>[6x]GPAGSMKPQIRNMVEPMDPRTFVSNFNNRPILSGLDTVWLCCEVKTKDPSGPPLDAKIFQGKVYPKAKYHPEMRFLRWFHKWRQLHHDQEYKVTWYVSWSPCTRCANSVATFLAKDPKVTLTIFVARLYYFWKPDYQQALRILAEAGATMKIMNYNEFQDCWNKFVDGRGKPFKPWNNLPKHYTLLQATLGELLRH

APOBEC3s (A3s) are deoxycytidine deaminases that have important roles in mammalian innate immune responses. Members of this family catalyze the conversion of cytosine into uracil on single-stranded DNA (ssDNA) and restrict retroviral replication and endogenous retroelements. Among all the A3s, A3G is most known for being a potent restriction factor against HIV-1. Similar to hA3G-CD1, rA3G-CD1 forms oligomers, binds to ssDNA/RNA strongly, and is catalytically inactive.

Here, we report the high-resolution (2 Å) crystal structure of a nearly wild-type (WT) A3G-CD1 from rhesus macaque (Macaca mulatta) (rA3G-CD1). We obtained two crystal forms of the rA3G-CD1 protein under different crystallization conditions, and determined the structures to 2 Å (CD1-1) in one crystal form and 2.9 Å (CD1-2) in the other crystal form, each in different space groups and with different crystal packing interactions. However, these two structures are essentially the same, with a Cα r.m.s. deviation of about 0.54 Å, indicating that the structures from the two different crystal forms, including the surface loops, are not affected by different crystal packing or buffer conditions. Therefore, the 2 Å high-resolution structure CD1-1 was used for structural analysis and comparison with other A3s, as similar results were also seen with the 2.9 Å resolution structure CD1-2. The 2 Å crystal structure of rA3G-CD1 indicates that the core structures of both the non-catalytic CD1 and the catalytic domains of A3s are highly conserved, including the Zn-centre conformation, the core β-strands, the N-terminal end of α2 and the orientations of α2–α4. Despite the close similarity of its core structure to other known A3 structures, rA3G-CD1 has a much more pronounced positively charged surface than any other A3. Interestingly, the positively charged residues of rA3G-CD1 are mainly distributed on one side of the molecule that is opposite the C terminus. Three major positively charged patches are formed around β2-loop-3-α2-α3 (Patch 1), loop-1-loop-7-α6 (Patch 2) and N-α1-loop-10 (Patch 3), respectively. The formation of the rA3G-CD1 dimer merges the positively charged patch 2 of the two CD1s and bridges the positively charged patch 1 and patch 3 on the same side of the dimer, generating a wide positively charged surface. In the crystal structure of rA3G-CD1, Y125, K128 and D130 are in close proximity, forming a compact charged interface around residue 128.>MSTVGTGKLTRAQRRAAARKNKRNTRVVQPVIVEPIASGQGKAIKAWTGYSVSKWTASCAAAEAKVTSAITISLPNELSSERNKQLKVGRVLLWLGLLPSVSGTVKSCVTETQTTAAASFQVALAVADNSKDVVAAMYP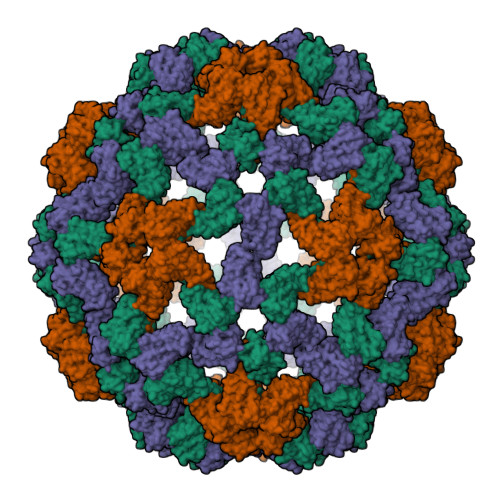EAFKGITLEQLTADLTIYLYSSAALTEGDVIVHLEVEHVRPTFDDSFTPVY[3x]>[2x]MRDLLSKKSHRQLELLELLFEHKRWFHRSELAELLNCTERAVKDDLSHVKSAFPDLIFHSSTNGIRIINTDDSDIEMVYHHFFKHSTHFSILEFIFFNEGCQAESICKEFYISSSSLYRIISQINKVIKRQFQFEVSL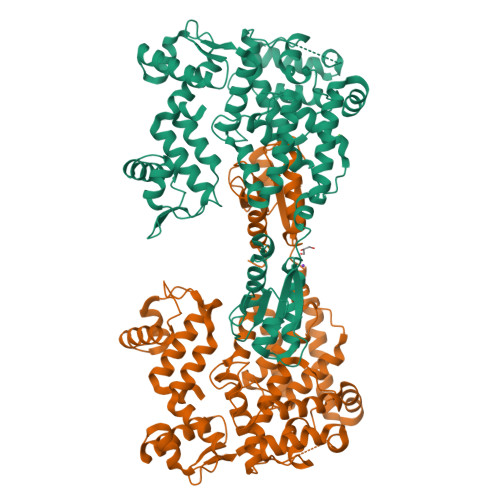TPVQIIGNERDIRYFFAQYFSEKYYFLEWPFENFSSEPLSQLLELVYKETSFPMNLSTHRMLKLLLVTNLYRIKFGHFMEVDKDSFNDQSLDFLMQAEGIEGVAQSFESEYNISLDEEVVCQLFVSYFQKMFFIDESLFMKCVKKDSYVEKSYHLLSDFIDQISVKYQIEIENKDNLIWHLHNTAHLYRQELFTEFILFDQKGNTIRNFQNIFPKFVSDVKKELSHYLETLEVCSSSMMVNHLSYTFITHTKHLVINLLQNQPKLKVLVMSNFDQYHAKFVAETLSYYCSNNFELEVWTELELSKESLEDSPYDIIISNFIIPPIENKRLIYSNNINTVSLIYLLNAMMFIRLDEAGHHHHHH> MAHHHHHHDYGIPTTENLYFQGSNPNYCFAGKTSSISDLKEVPRKNITLIRGLGHGAFGEVYEGQVSGMPNDPSPLQVAVKTLPEVCSEQDELDFLMEALIISKFNHQNIVRCIGVSLQSLPRFILMELMAGGDLKSFLRETRPRPSQPSSLAMLDLLHVARDIACGCQYLEENHFIHRDIAARNCLLTCPGPGRVAKIGDFGMARDIYRASYYRKGGCAMLPVKWMPPEAFMEGIFTSKTDTWSFGVLLWEIFSLGYMPYPSKSNQEVLEFVTSGGRMDPPKNCPGPVYRIMTQCWQHQPEDRPNFAIILE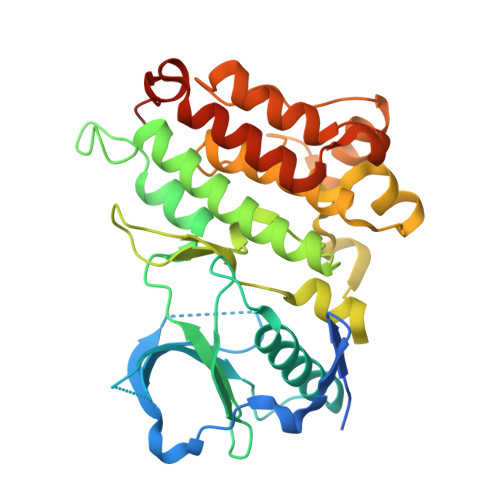RIEYCTQDPDVINTALPIEYGPLVEEEEKV> MGHHHHHHGSLVPRGSDVQELNSIIQRISKFDNILKDKTIINQQDLRQISWNGIPKIHRPVVWKLLIGYLPVNTKRQEGFLQRKRKEYRDSLKHTFSDQHSRDIPTWHQIEIDIPRTNPHIPLYQFKSVQNSLQRILYLWAIRHPASGYVQGINDLVTPFFETFLTEYLPPSQIDDVKIKDPSTYMVDEQITDLEADTFWCLTKLLEQITDNYIHGQPGILRQVKNLSQLVKRIDADLYNHFQNEHVEFIQFAFRWMNCLLMREFQMGTVIRMWDTYLSETSQEVTSSYSMSSNDIKPPVTPTEPRVASFVTPTKDFQSPTTALSNMTPNNAVEDSGKMRQSSLNEFHVFVCAAFLIKWSDQLMEMDFQETITFLQNPPTKDWTETDIEMLLSEAFIWQSLYKDATSHWL;> MGHHHHHHGSSSCAVSGASGCLPPARSRIFKIIVIGDSNVGKTCLTYRFCAGRFPDRTEATIGVDFRERAVDIDGER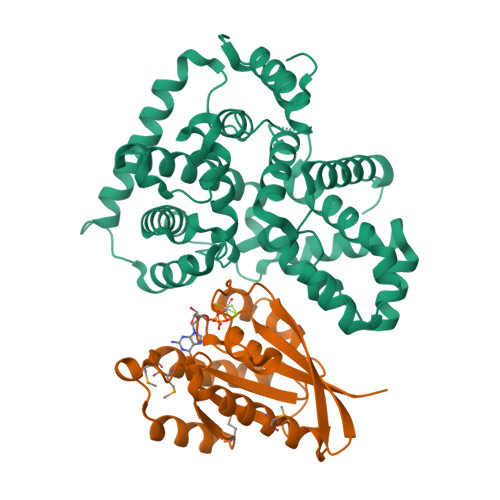IKIQLWDTAGQERFRKSMVQHYYRNVHAVVFVYDMTNMASFHSLPAWIEECKQHLLANDIPRILVGNKCDLRSAIQVPTDLAQKFADTHSMPLFETSAKNPNDNDHVEAIFMTLAHKLKSH> GAEISTFPHSGLSYPDINFKIF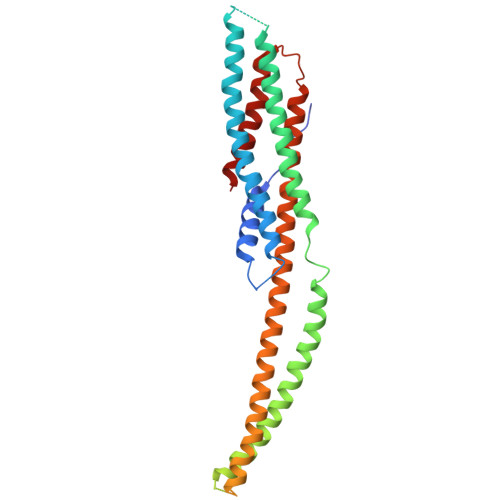SQGVKNISHLAQFKTTGVEVLQEKALRVSLYSQRLDVIVRESLSSLQVKLENTLALTYFTTLEEIDEALISQDIDEESKSEMRKERINIIKNLSNDITQLKQLFIEKTELLDKSSSDLHNVVIIEGTDKVLQAEQLRQKQLTEDIATKELERKEIEKKRDKIIEALDVIREHNLVDAFKDLIPTGENLSELDLAKPEIELLKQSLEITKKLLGQFSEGLKYIDLTDARKKLDNQIDTASTRLTELNRQLEQSEKLIAGVNAVIKIDQEKSAVVVEAEKLSRAWHIFIHEITALQGTSLNEVELSKPLIKQQIYLESLIKQLI>[2x]MRVLITGCGSRGDTEPLVALAARLRELGADARMCLPPDYVERCAEVGVPMVPVGRAVRAGAREPGELPPGAAEVVTE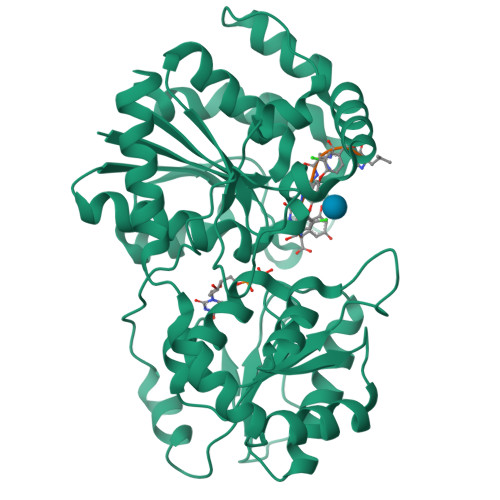VVAEWFDKVPAAIEGCDAVVTTGLLPAAVAVRSMAEKLGIPYRYTVLSPDHLPSEQSQAERDMYNQGADRLFGDAVNSHRASIGLPPVEHLYDYGYTDQPWLAADPVLSPLRPTDLGTVQTGAWILPDERPLSAELEAFLAAGSTPVYVGFGSSSRPATADAAKMAIKAVRASGRRIVLSRGWADLVLPDDGADCFVVGEVNLQELFGRVAAAIHHDSAGTTLLAMRAGIPQIVVRRVVDNVVEQAYHADRVAELGVGVAVDGPVPTIDSLSAALDTALAPEIRARATTVADTIRADGTTVAAQLLFDAVSLEKPTVPALEHHHHHH> GGGRQPFNFEGLDIPVYFIDKPYSELASSVELSFVNDDSPLLFPEMDSRLPKPTPELDIKYYSSNLSSFKEDTVILMRGTTEEEAWNIANYKTAGGSNK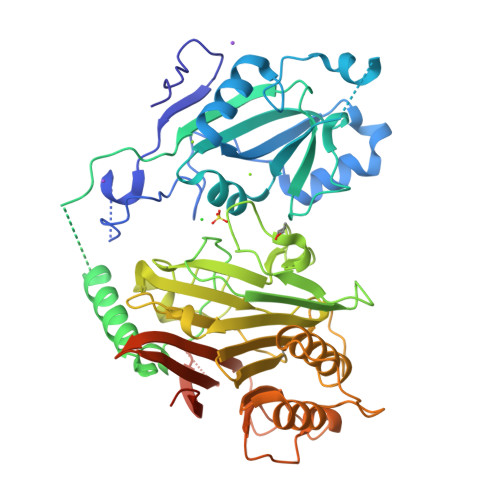DLEENFIEAGPQFNLSFSEYTSSINSADTASRKHFLVIIKVQVKYISNDNVLYANHWAIPDEAPVEVLAVVDRRFIFPEPPVKPKLSFIQKIANRFLTENVAEISSINFRRLNSGNINVLKGRGVFSSRRLREIYLRFDAANADELRPGDVYVKKTKFDSMGYDSHFYNEGIGINGAPTLNTYTGEYVADSSSQGATYWLKYNLTNETSIIKVSNSARGANGIKIALEEIEENKPVVITSGTLTGCTVVFARKGEYFYAVHTGNSESLIGFTSTSGVAKAIEVLSSLSELEVPALPDVINNNTLVEYLSDNFDSALISYSSSSLKPNSMINISRENVSTFSYYTDDIQLPSFGTSVTILVRTNDNTVVRSLSESYTMNSNSSKMVVFNVLQKDFSAGGDYKDHDGDYKDHDIDYKDDDDK> GSHMASMFGKLREKLKSFVKRVEEEVEKEEEEVEKKGLLDRILTVEIKEKDVDKALDELEIDLLEADVALEVVDALREKIKQKLVGKKVRIGTDKGKIIEEAVKEAVSEILETSRRIDLIEEIRKAEKPYVIMFVGFNGSGKTTTIAKLANWLKNHGFSVVIAASDTFRAGAIEQLEEHAKRIGVKVIKHSYGADPAAVAYDAIQHAKARGIDVVLIDTAGRSETNRNLMDEMKKIARVTKPNLVIFVGDALAGNAIVEQARQFNEAVKIDGIILTKLDADARGGAALSI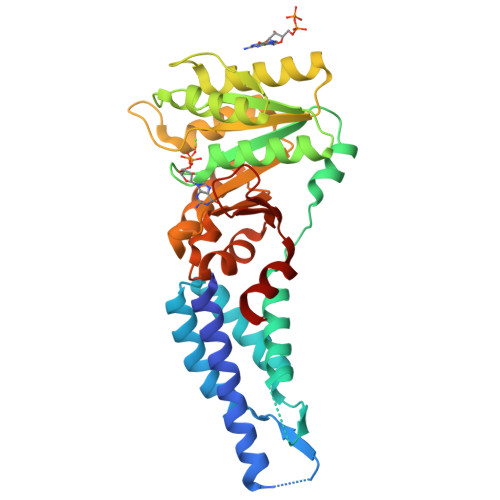SYVIDAPILFVGVGQGYDDLRPFEKEWFLERIFGEENA> QYSSNTQQGRTSIVHLFEWRWVDIALECERYLAPKGFGGVQVSPPNENVAIHNPFRPWWERYQPVSYKLCTRSGNEDEFRNMVTRCNNVGVRIYVDAVINHMCGNAVSAGTSSTCGSYFNPGSRDFPAVPYSGWDFNDGKCKTGSGDIENYNDATQVRDCRLSGLLDLALGKDYVRSKIAEYMNHLIDIGVAGFRIDASKHMWPGDIKAILDKLHNLNSNWFPEGSKPFIYQEVIDLGGEPIKSSDYFGNGRVTEFKYGAKLGTVIRKWNGEKMSYLKNWGEGWGFMPSDRALVFVDNHDNQRGHGAG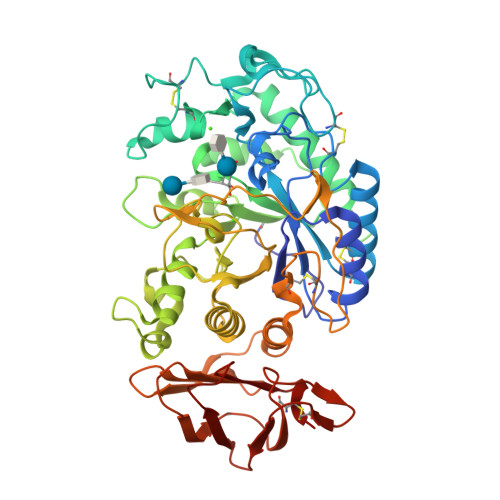GASILTFWDARLYKMAVGFMLAHPYGFTRVMSSYRWPRYFENGKDVNDWVGPPNDNGVTKEVTINPDTTCGNDWVCEHRARQIRNMVNFRNVVDGQPFTNWYDNGSNQVAFGRGNRGFIVFNNDDWTFSLTLQTGLPAGTYCDVISGDKINGNCTGIKIYVSDDGKAHFSISNSAEDPFIAIHAESKL>GAMGSMATYEVLCEVAEKLGTDDREVVLFLLNVFIPQPTLAQLIGALRALKEEGRLTFPLLAECLFRAGRRDLLRDLLHLDPRFLERHLAGTMSYFSPYQLTVLHVDGELCARDIRSLIFLSKDTIGSRSTPQTFLHWVYCMENLDLLGPTDVDALMSMLRSLSRVDLQRQVQTLMGLHLSGPSHSQHYRHTP[6x]

Pivotal to the survival of both tumors is the canonical NF-κB pathway that becomes constitutively activated by the virally encoded protein vFLIP. In contrast to the ubiquitin-dependent mechanisms, persistent IKK kinase activation by vFLIP proceeds via a direct association between vFLIP and IKKγ. Taken together, our results are the first to reveal that vFLIP-induced NF-κB activation pivots on the formation of structurally specific vFLIP–IKKγ multimers which have an important role in rendering the kinase subunits active through a process of autophosphorylation. Key to the formation of oligomeric vFLIP–IKKγ assemblies are interactions contributed by amino acids R12 and E104 in vFLIP.

An R12E vFLIP mutant was generated to maximally disrupt the vFLIP–IKKγ interactions and a D102R E104R vFLIP double mutant to disrupt vFLIP–vFLIP contacts. All were observed to have a similar elution profile during SEC MALS to that of WT vFLIP with the exception of R12E. Rather than eluting predominantly as a monomer (preceded by a small dimer peak), the R12E mutant had an enhanced dimeric component comparable to that of the monomer in terms of UV absorbance (left). The tendency of this mutant to dimerize was confirmed by native mass spectrometry and shown to be reducing agent dependent since treatment with 10 mM TCEP resulted in a shift to a predominant monomer when re-investigated using SEC (right). These observations could be explained by the crystal structure of the R12E mutant that was refined to 4.2 Å. In this structure, six R12E monomers form the asymmetric unit, two of which appear to be appropriately positioned for formation of a disulfide bridge mediated by C106, in an extended but weakly stabilized interface that also incorporates E12 and K13. Furthermore, ITC experiments confirmed that the R12E mutant had a similar Kd to that of WT vFLIP consistent with previous reports and the high levels of similarity between the R12E vFLIP and WT vFLIP co-ordinates in the vFLIP–IKKγ(150–272) complex when superposed. Whilst all mutants appeared unimpaired in their capacity to associate with IKKγ following immunoprecipitation consistent with our biochemical and biophysical assays and were expressed at similar levels, R12E displayed significant reductions in its capacity to phosphorylate GST-IκBα(1–54) and NF-κB activation. Although the D102R E104R mutant was the least disrupted and had a near WT elution profile, the R12E mutant lacked a defined hetero-octamer peak that was instead replaced by a broad range of interchanging higher molecular species extending from the hetero-octamer region almost to the void of the column. The fact that the R12E mutant appears capable of forming higher order species based on our SEC data, the lack of a clearly defined hetero-octamer coupled with the defective oligomerization observed in blue native gels suggests that the vFLIP–IKKγ assemblies capable of activating the IKK kinase are structurally specific.> HHHHHHMSLRKQRFMQFSSLEHEGEYYMTPRDFLFSVMFEQMERKTSVKKLTKKDIEDTLSGIQTAGCGSTFFRDLGDKGLISYTEYLFLLTILTKPHSGFHVAFKMLDTDGNEMIEKREFFKLQKIISKQDDLMTVKTNETGYQEAIVKEPEINTTLQMRFFGKRGQRKLHYKEFRRFMENLQTEIQEMEFLQFSKGLSFMRKEDFAEWLLFFTNTENKDIYWKNVREKL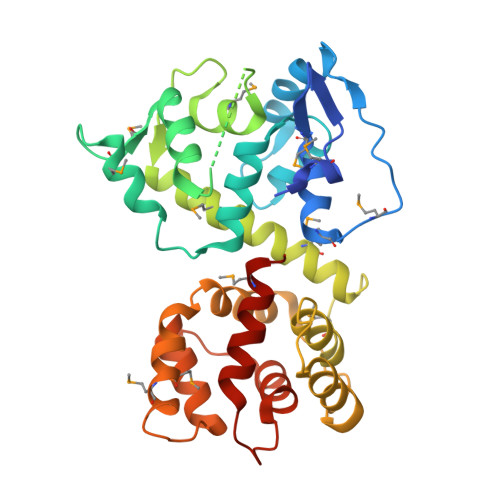SAGESISLDEFKSFCHFTTHLEDFAIAMQMFSLAHRPVRLAEFKRAVKVATGQELSNNILDTVFKIFDLDGDECLSHEEFLGVLKNRMHRGLWV>[6x]MAVEEIVKVSRNYQVTIPAKVRQKFQIKEGDLVKVTFDESEGVVKIQL

Sso7c4 appears to be the first repressor-like protein described in crenarchaea and may play a regulatory role in gene transcription. The Sso7c4 protein possesses a homodimeric DNA-binding fold that forms a swapped β-loop-β ‘Yin-Yang’ topology, and it belongs to the SpoVT-AbrB superfamily. The dimeric Sso7c4 protein, which consists of eight intertwined β sheets and two flanking α helices, forms a dimer via intermolecular associations between β1 and β3′ (the primes indicate the second monomer in the dimer) and β1′ and β3 in the flank, β2 and β2′ at the top, and β4 and β4′ at the bottom. In our study, Sso7c4 exhibits DNA-binding activity and alters the trajectory of the DNA through bending and bridging.

We also determined the crystal structure of C-terminally truncated Sso7c4 at a resolution of 1.4 Å to address the potential effect of the flexible C-terminus on DNA binding. In contrast to the wild-type structure, there are three homodimers in one asymmetric unit of the C-terminally truncated Sso7c4 crystal, which is in the P31 space group. The crystal structures of the wild-type and C-terminally truncated proteins are similar, as indicated by the good superposition of their α carbons (the r.m.s.d. value is 0.35 Å for 85 atoms). In the crystal structure of the C-terminal truncation mutant, the R11 side chains of the three molecules in one asymmetric unit are all exposed to solvent and flexible, consistent with the results of previous NMR dynamics studies. The FP results showed that all the C-terminally truncated proteins exhibited lower binding affinity to 8-bp, 10-bp, and 20-bp DNAs than the wild-type protein. In contrast, the C-terminally truncated protein bound to the 10-bp and 20-bp DNAs with similar affinities (~11 μM) but bound to the 8-bp DNA with slightly weaker affinity. At higher protein:DNA ratios (1:0.5 dimer:bp), a considerable number of C-terminally truncated Sso7c4-DNA complexes were observed to form a more open circular shape (67%, n = 109), suggesting that the C-terminally truncated proteins induced DNA stiffening. However, the DNA contour length was not reduced upon C-terminally truncated Sso7c4 binding (1834.97 nm for 5 bp/dimer and 1830.06 nm for 0.5 bp/dimer), implying that both C-termini of Sso7c4 are also involved in bending DNA. The FRET data confirm the EM observation showing that the C-terminally truncated protein forms a rigid filament along DNA. In conclusion, wild-type Sso7c4 induces the formation of a more compact DNA structure primarily through both bridging and bending interactions, whereas C-terminally truncated proteins rigidify and open the DNA molecules at high protein concentrations.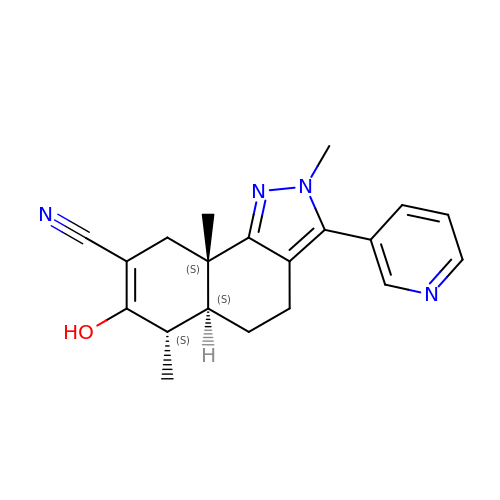(5aS,6S,9aS)-7-hydroxy-2,6,9a-trimethyl-3-(pyridin-3-yl)-4,5,5a,6,9,9a-hexahydro-2H-benzo[g]indazole-8-carbonitrile | C20 H22 N4 O | IQRJTLOGKWCNQB-APXLUKDGSA-N> CCACUGAGAGC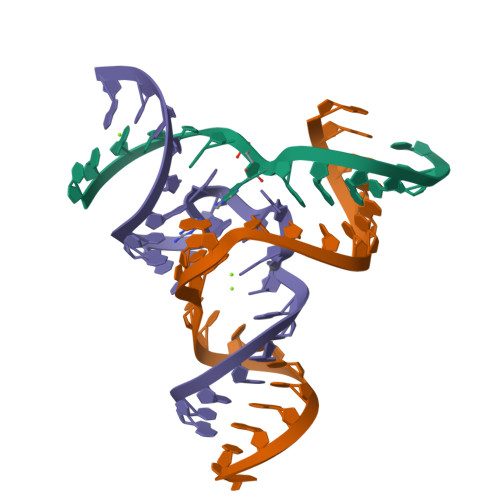UUC;> GGAAGCUCUGACCGACCCCCAGCC;> GCUGGGACAACUAGACAUACAGUG> SPMSATALLQKAAQMGS;> GPMVAMFQEDNGTSSVASSPLQVFSTMSLNRPTLLASSSPFHCLKDLKPEERGLYLIHLLLTCANHVASGSLQNANAALEQLSHLASPDGDTMQRIAAYFTEALANRILKSWPGLYKALNATQTRTNNVSEEIHVRRLFFEMFPILKVSYLLTNRAILEAMEGEKMVHVIDLDASEPAQWLALLQAFNSRPEGPPHLRITGVHHQKEVLE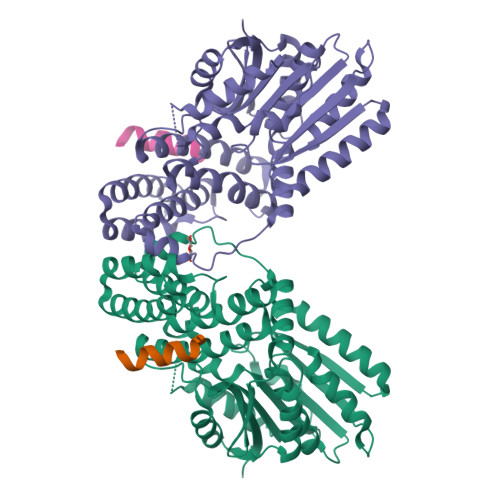QMAHRLIEEAEKLDIPFQFNPVVSRLDCLNVEQLRVKTGEALAVSSVLQLHTFLASDDDLMRKNCALRFQNNPSGVDLQRVLMMSHGSAAEARENDMSNNNGYSPSGDSASSLPLPSSGRTDSFLNAIWGLSPKVMVVTEQDSDHNGSTLMERLLESLYTYAALFDCLETKVPRTSQDRIKVEKMLFGEEIKNIISCEGFERRERHEKLEKWSQRIDLAGFGNVPLSYYAMLQARRLLQGCGFDGYRIKEESGCAVICWQDRPLYSVSAWRCRK> TGGGGGTTTGGGGGTTTGGGG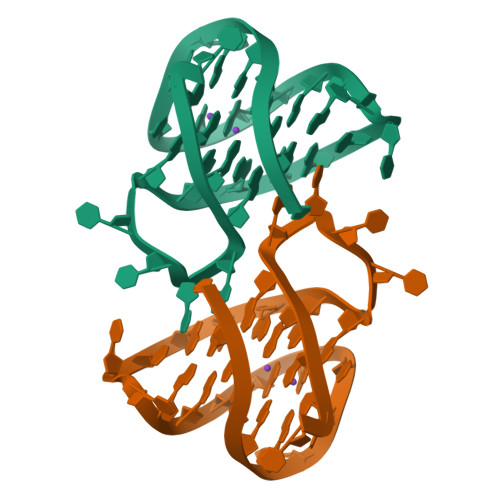GTTTGGGGGT> MADLNWMQRGVRAVELNVAARLENLALLRTLVGAIGTFEDLDFDAVADLRLAVDEVCTRLIRSALPDATLRLVVDPRKDEVVVEASAACDTH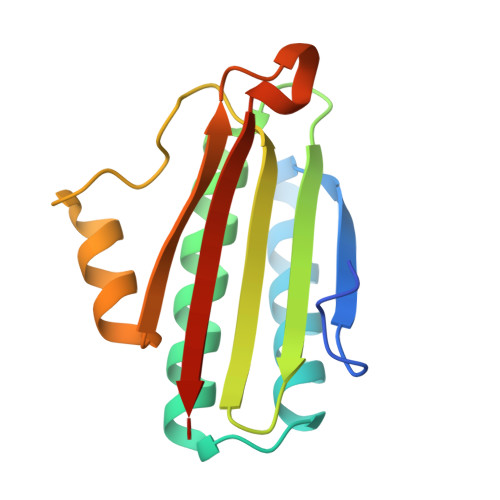DVVAPGSFSWHVLTALADDVQTFHDGRQPDVAGSVFGITLTARRAASSR> MSKEQLLIQRSSAAERCRRYRQKMSAEQRASDLERRRRLQQNVSEEQLLEKRRSEAEKQRRHRQKMSKDQRAFEVERRRWRRQNMSREQSSTSTTNTGRNCLLSKNGVHEDAILEHSCGGMTVRCEFCLSLNFSDEKPSDGKFTRCCSKGKVCPNDIHFPDYPAYLKRLMTNEDSDSKNFMENIRSINSSFAFASMGANIASPSGYGPYCFRIHGQVYHRTGTLHPSDGVSRKFAQLYILDTAEATSKRLAMPENQGCSERLMININNLMHEINELTKSYKMLHEVEKEAQSEAAAKGIAPTEVTMAIKYDRNSDPGRYNSPRVTEVAVIFRNEDGEPPFERDLLIHCKPDPNNPNATKMKQISILFPTLDAMTYPILFPHGEKGWGTDIALRLRDNSVIDNNTRQNVRTRVTQMQYYGFHLSVRDTFNPILNAGKLTQQFIVDSYSKMEANRINFIKANQSKLRVEKYSGLMDYLKSRSENDNVPIGKMIILPSSFEGSPRNMQQRYQDAMAIVTKYGKPDLFITMTCNPKWADITNNLQRWQKVENRPDLVARVFNIKLNALLNDICKFHLFGKVIAKIHVIEFQKRGLPHAHILLILDSESKLRSEDDIDRIVKAEIPDEDQCPRLFQIVKSNMVHGPCGIQNPNSPCMENGKCSKGYPKEFQNATIGNIDGYPKYKRRSGSTMSIGNKVVDNTWIVPYNPYLCLKYNCHINVEVCASIKSVKYLFKYIYKGHDCANIQISEKNIINHDEVQDFIDSRYVSAPEAVWRLFAMRMHDQSHAITRLAIHLPNDQNLYFHTDDFAEVLDRAKRHNSTLMAW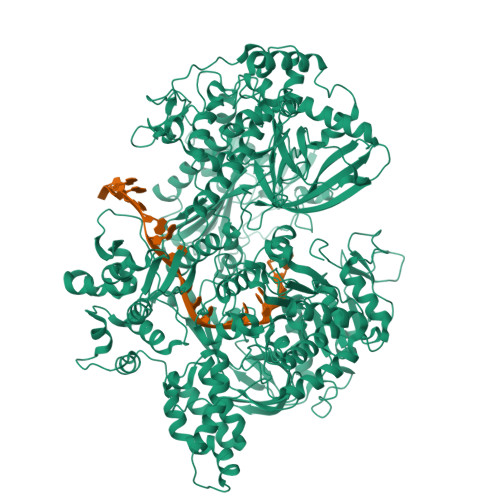FLLNREDSDARNYYYWEIPQHYVFNNSLWTKRRKGGNKVLGRLFTVSFREPERYYLRLLLLHVKGAISFEDLRTVGGVTYDTFHEAAKHRGLLLDDTIWKDTIDDAIILNMPKQLRQLFAYICVFGCPSAADKLWDENKSHFIEDFCWKLHRREGACVNCEMHALNEIQEVFTLHGMKCSHFKLPDYPLLMNANTCDQLYEQQQAEVLINSLNDEQLAAFQTITSAIEDQTVHPKCFFLDGPGGSGQTYLYKVLTHYIRGRGGTVLPTASTGIAANLLLGGRTFHSQYKLPIPLNETSISRLDIKSEVAKTIKKAQLLIIDECTMASSHAINAIDRLLREIMNLNVAFGGKVLLLGGDFRQCLSIVPHAMRSAIVQTSLKYCNVWGCFRKLSLKTNMRSEDSAYSEWLVKLGDGKLDSSFHLGMDIIEIPHEMICNGSIIEATFGNSISIDNIKNISKRAILCPKNEHVQKLNEEILDILDGDFHTYLSDDSIDSTDDAEKENFPIEFLNSITPSGMPCHKLKLKVGAIIMLLRNLNSKWGLCNGTRFIIKRLRPNIIEAEVLTGSAEGEVVLIPRIDLSPSDTGLPFKLIRRQFPVMPAFAMTINKSQGQTLDRVGIFLPEPVFAHGQLYVAFSRVRRACDVKVKVVNTSSQGKLVKHSESVFTLNVVYREILE Rai1 homologs share several highly conserved sequence motifs, and our structural studies show that they are located in the active site region, mediating the binding of the divalent metal ions and/or the RNA. We have found substantial variations in the activity profiles of the Rai1 homologs, and discovered that some of them possess a new 5′ triphosphonucleotide hydrolase (TPH) activity. The overall structures of CaRai1, AgRai1 and SsRai1 are similar to those of SpRai1 (16), KlDxo1 (18), and MmDXO. Each structure contains two mixed β-sheets that are surrounded by α-helices.

The AgRai1–pU(S)6–Mn2+ complex was prepared by soaking AgRai1 free enzyme crystals with 10 mM pU(S)6 and 10 mM MnCl2 overnight. Clear electron density was observed for all six nucleotides of the RNA in the AgRai1–pU(S)6–Mn2+ ternary complex. The structure reveals that pU(S)6 is also bound as a product to the active site of AgRai1, with its 5′ phosphate being a bridging ligand to both Mn2+ ions, in contrast to our observations with MmDXO where the binding mode of pU(S)6 mimics the substrate. There is also a third Mn2+ near the active site, but its position is 3.3 Å from that observed in CaRai1 and it interacts with the protein through its coordinating water molecules. The first two nucleotides of pU(S)6 make conserved interactions with AgRai1. The backbone phosphorothioate group of the third nucleotide, U4, interacts with Lys254 (motif V) but is about 5 Å away from Arg275 (motif VI). The positions of its ribose and base show clear differences to those of U4 in the MmDXO complex, probably because the side chain of Trp154 (αD) in AgRai1 clashes with the position of U4 in the MmDXO complex. While the five bases of pU5 in the MmDXO complex maintain base stacking, the last two bases of pU(S)6 in the AgRai1 complex are flipped relative to the first four bases, and the last base is positioned against the side chain of Asn253 (αF), at the opening of the active site pocket. We also observed a sulfate or phosphate ion (modeled as sulfate) in the active site region of this structure, bound through interactions with the dipole of helix αB (backbone amides of Arg106 and Gly107), the side chain guanidinium group of Arg106 (motif I), and the side chain ammonium ion of Lys198 (β9). Three residues were found to be located near pU(S)6 that are present almost exclusively in AgRai1: Lys110 (αB, interacting with the base of U5), Trp154 (αD, near U4) and Tyr159 (αD, near U2 base).

>MVFESELLLQRRLATTALKQPKELGYYSTNVGGELKVMDESNLSYYYLPDADIEKHIDLSAGARKFQDEQAEAEDDTGSLHGLLQTLMEYERRKSKKVNADIIAFRGQVKRLIHCAFGGHATDVDMYVMSFDGQLFIRAARKKLEFPTSPRESWAYLAYYSGYKFERMALLDRPVAETPREVLESRGKQVVRNGPQYKTVVRTGVGEHKLVLGAEVDGIFDFREPTGDNLKHYVELKVAKKVQTLKDATNFEQKLFSVWLQCFLVGINRVIIGFRDEKFVLKSVEEFSTSEIPLLLKSTGLRNACVDAIKWYGALTKWLCELPRGPEDDFKLYRLSCSRGALHLRQLHDEDLANGDDIIPGWFREWRRSLSKSHGS[2x]> MAGNFWQSSHYLQWILDKQDLLKERQKDLKFLSEEEYWKLQIFFTNVIQALGEHLKLRQQVIATATVYFKRFYARYSLKSID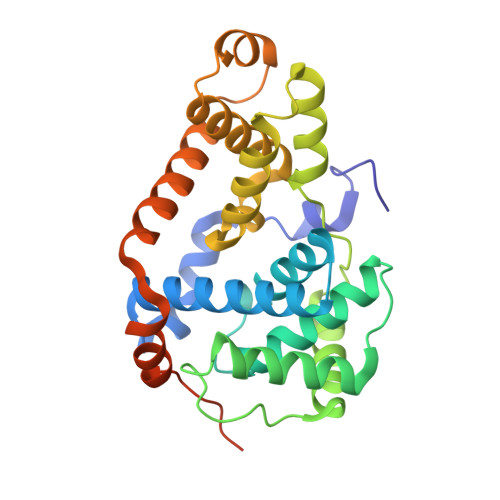PVLMAPTCVFLASKVEEFGVVSNTRLIAAATSVLKTRFSYAFPKEFPYRMNHILECEFYLLELMDCCLIVYHPYRPLLQYVQDMGQEDMLLPLAWRIVNDTYRTDLCLLYPPFMIALACLHVACVVQQKDARQWFAELSVDMEKILEIIRVILKLYEQWKNFDERKEMATILSKMPKPKPPPNSEGEQGPNGSQNSSYSQS> GPHMKFTVEREHLLKPLQQVSGPLGGRPTLPILGNLLLQVADGTLSLTGTDLEME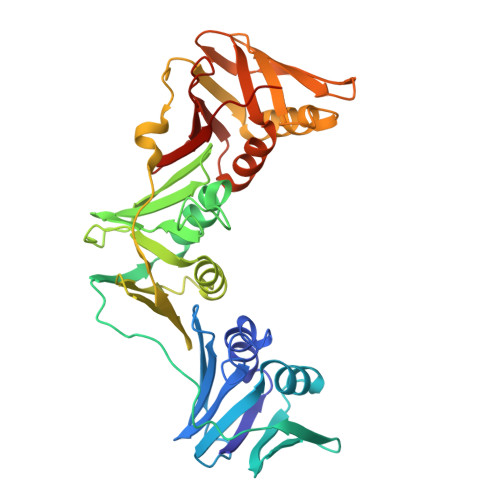MVARVALVQPHEPGATTVPARKFFDICRGLPEGAEIAVQLEGERMLVRSGRSRFSLSTLPAADFPNLDDWQSEVEFTLPQATMKRLIEATQFSMAHQDVRYYLNGMLFETEGEELRTVATDGHRLAVCSMPIGQSLPSHSVIVPRKGVIELMRMLDGGDNPLRVQIGSNNIRAHVGDFIFTSKLVDGRFPDYRRVLPKNPDKHLEAGCDLLKQAFARAAILSNEKFRGVRLYVSENQLKITANNPEQEEAEEILDVTYSGAEMEIGFNVSYVLDVLNALKCENVRMMLTDSVSSVQIEDAASQSAAYVVMPMRL>[2x]GSGTMKFAEHLSAHITPEWRKQYIQYEAFKDMLYSAQDQAPSVEVTDEDTVKRYFAKFEEKFFQTCEKELAKINTFYSEKLAEAQRRFATLQNELQSSGSGSGDLKLAFSEFYLSLIL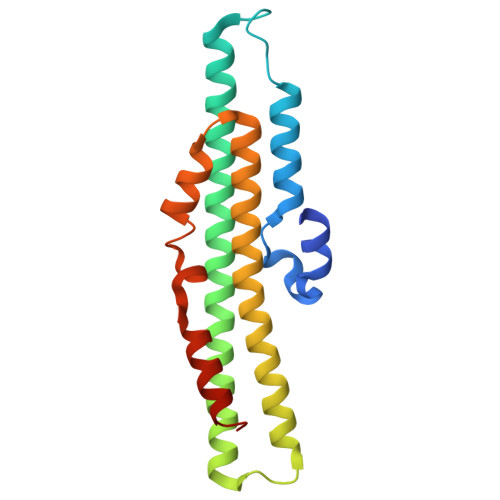LQNYQNLNFTGFRKILKKHDKILETSRGADWRVAHVEVAPFYTCKKINQLISETEAVVTNELE> MSNQTDADVIVIGAGPSGSYAAKLLHDQGVRVKLVEAKDRVGGRTWSTKSDAPGGPIDFGGQWIGETHVLLPELGAELGLETVSSVKPGNDLFVFNGDVEVGEEDQVPSGASWAGELSRSFELLDEVGTRLGWAAPWASEHVGELDSMTVAQWLEQNVQSSEVRLIHEVMVNILNGASTTEVSMAYWAYFVHQGEGIESLIGTRSGAQVAWFIGGMGQVTELIADKLGDDVHLNWPVTRIEQDPTGVTVFSGERRLRASFAILAAPPSAGSRMIFDPPLPPKRAQLQARAPMGRLAKIQVRYDEPFWQERGLSGAAFECGDLAFWLFDGSKPTDSLATIVGFIGGKHLDAWHALSPNEREKRFIEILVNNFGDKARDVRYVHETDWTVQPWTGGAPVTFMPTG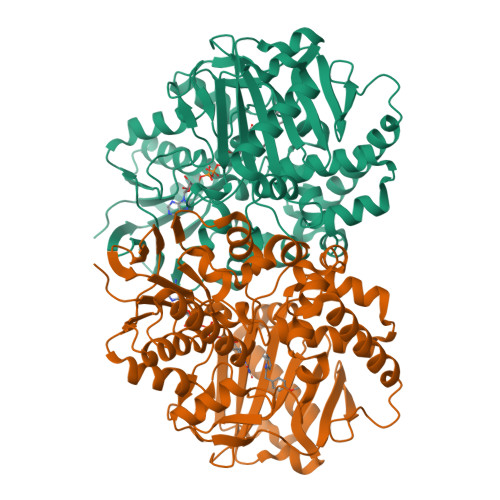LLSSAGSALREPVDRLHFAGTEAAPMWSGYIEGALRAGKIAAGDVLARLA> MAHHHHHHMGTNKPFVVVVDDDASVGRAIRRLLRSVGIAADTYTSGDEFLDVLSATPS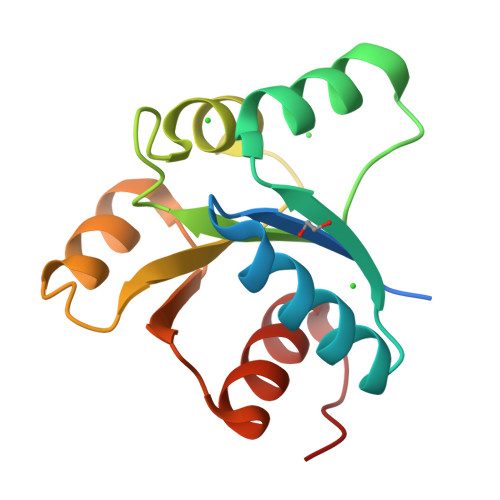YRPDCVILDVQMPGSNGIEVQRRLAGGAVPVIFITAHDDAGVRETALAAGARAYLRKPFNDVLFIRTVCAVLGIAAPL N6-BENZYL-NICOTINAMIDE-ADENINE-DINUCLEOTIDE 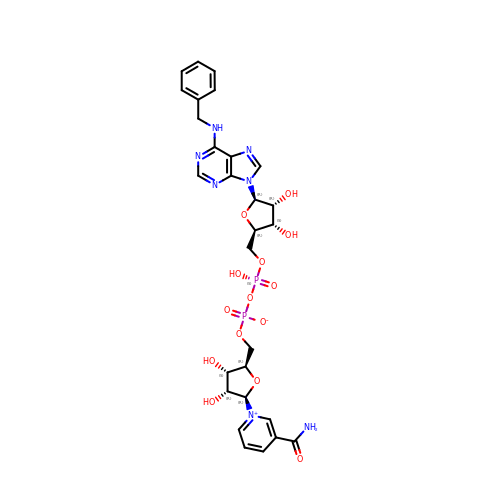| C28 H33 N7 O14 P2 | PDNSIRRMIDXSBH-INGGVVRRSA-N>SNANDTDGDTLDVLLPLRTTGEKAPLFCVHPAGGLSWVYSGLMQHIGADRPLYGLQARGLADPSATLPSSIEEMAADYVTQIRGVQPSGPYHLLGWSLGSLVIHAMATQLRAEGEEVGLLVNLDQYPIDRSRPAPESQPDQQDALRIMLDFVGYDMDSLGDEPLDYAMVADVLRERQSVFANLDETAITALANVFANSRSLFGSFAPQPLDSDVLVIVAEP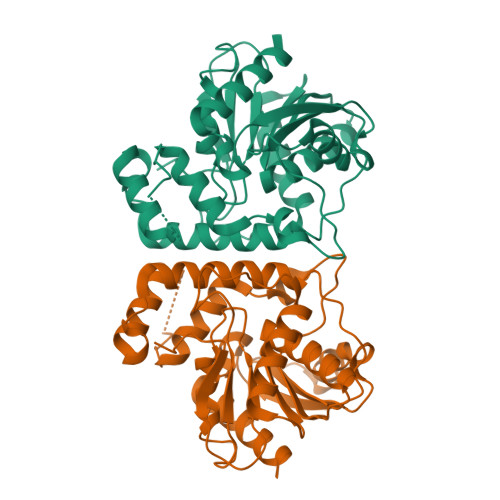DETVPAAELAARVEQWRPFVTGKIEYQTVRCSHPHMMQPEPAAEIGRLIAEKLGTSK[3x]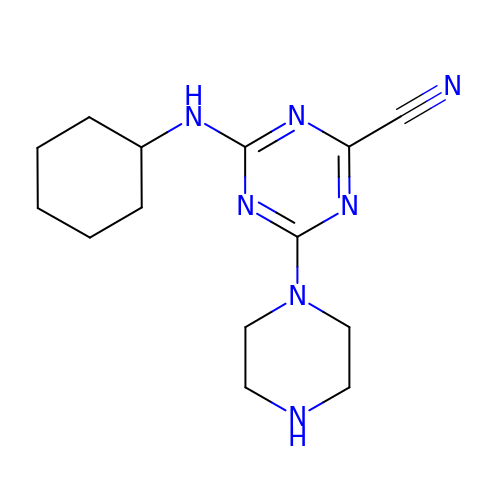4-(cyclohexylamino)-6-piperazin-1-yl-1,3,5-triazine-2-carbonitrile | C14 H21 N7 | ZBLLHXCRPWKVCY-UHFFFAOYSA-N ADARs (adenosine deaminases that act on RNA) catalyze adenosine deamination within duplex RNA yielding inosine. ADARs are multidomain proteins with N-terminal double stranded RNA binding domains (dsRBDs) and C-terminal deaminase domains. Since the substrate for ADARs is an RNA duplex, the enzymes access the reactive adenosine using a base flipping mechanism. For instance, the nearest neighbor nucleotide preferences for ADARs show a strong bias against reaction at adenosines with a guanosine 5′ to the target adenosine (5′-GA sites).

Therefore, we prepared a 32 bp duplex bearing azaN adjacent to a 5′ G paired with 3-deaza dA for X-ray crystallography with ADAR2-R2D E488Q. Crystals of this complex formed readily and diffracted X-rays beyond 2.8 Å. The overall structure of the asymmetric homodimeric protein bound to RNA is very similar to the structure described above (rmsd of 0.201 Å for 698 equivalent α-carbons) with well-resolved electron density for the purine:purine pair adjacent to the azaN. The G on the 5′ side of the azaN is in a syn conformation with its Hoogsteen face directed toward the Watson–Crick face of the 3-deaza dA on the opposing strand. The position of the substrate strand is shifted slightly from that of the structure described above such that, in this structure, the base pair hydrogen bonding involves 3-deaza dA N1 to G N7 (2.8 Å) and 3-deaza dA 6-amino to G O6 (3.0 Å). Interestingly, the shift in substrate RNA strand position observed in this Gsyn:AH+anti structure allows it to adopt a phosphodiester backbone conformation that is nearly identical to that seen in complexes with RNA bearing ADARs’ preferred 5′ nearest neighbor (5′ U paired with A). The standard conformation of this phosphate in the G:3-deaza dA pair might contribute to the observed higher deamination rate relative to the G:G pair.

>GASLAQPPLPVLPPFPPPSGKNPVMILNELRPGLKYDFLSESGESHAKSFVMSVVVDGQFFEGSGRNKKLAKARAAQSALAAIFNLHLDQTPSRQPIPSEGLQLHLPQVLADAVSRLVLGKFGDLTDNFSSPHARRKVLAGVVMTTGTDVKDAKVISVSTGTKCINGEYMSDRGLALNDCHAEIISRRSLLRFLYTQLELYLNNKDDQKRSIFQKSERGGFRLKENVQFHLYISTSPCGDARIFSPHEPILEEPADRHPNRKARGQLRTKIESGQGTIPVRSNASIQTWDGVLQGERLLTMSCSDKIARWNVVGIQGSLLSIFVEPIYFSSIILGSLYHGDHLSRAMYQRISNIEDLPPLYTLNKPLLSGISNAEARQPGKAPNFSVNWTVGDSAIEVINATTGKDELGRASRLCKHALYCRWMRVHGKVPSHLLRSKITKPNVYHESKLAAKEYQAAKARLFTAFIKAGLGAWVEKPTEQDQFSLTP[2x]>LKESPSGYLRSGEGDTGCGELVWVGEPLTLRTAETITGKYGVWMRDPKPTYPYTQETTWRIDTVGTDVRQVFEYDLISQFMQGYPSKVHILPRPLESTGAVVYSGSLYFQGAESRTVIRYELNTETVKAEKEIPGAGYHGQFPYSWGGYTDIDLAVDEAGLWVIYSTDEAKGAIVLSKLNPENLELEQTWETNIRKQSVADAFIICGTLYTVSSYTSADATVNFAYDTGTGISKTLTIPFKNRYKYSSMIHYNPLEKKLFAWDNLNMVTYDIKL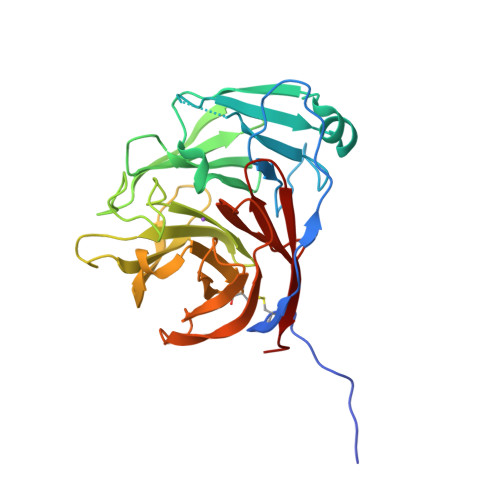SKM[2x]methyl 4-chloranyl-2-cyclohexylsulfanyl-5-sulfamoyl-benzoate 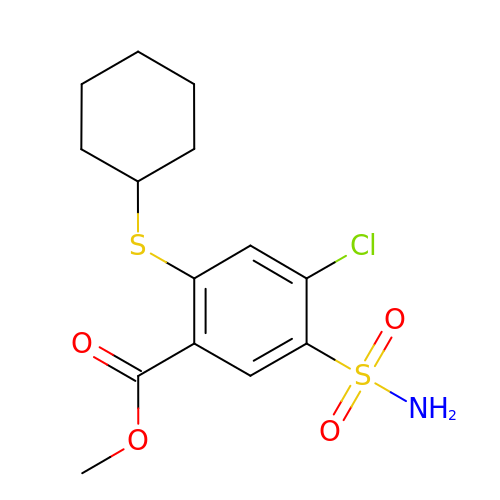| C14 H18 Cl N O4 S2 | PURDMVQHUYFOQM-UHFFFAOYSA-N[5-methoxy-2-({[2-nitro-4-(trifluoromethyl)phenyl]sulfonyl}carbamoyl)-1H-indol-1-yl]acetic 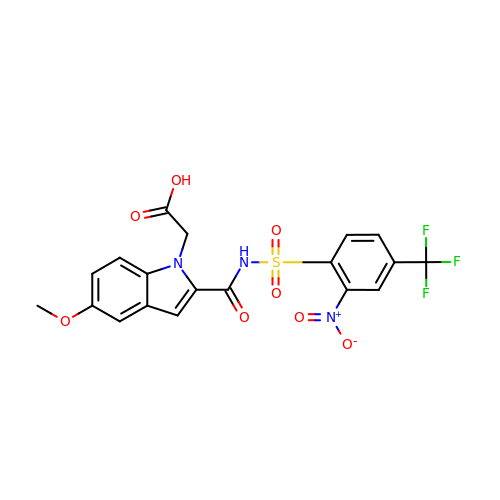acid | C19 H14 F3 N3 O8 S | PCVZSEOYPYERFT-UHFFFAOYSA-N> SNASFRVVLDPGHGGIDGGARGVTGILEKDVTLAFARALRDELQKGSHTIVALTRDSDIFLRLSERVKKAQEFDADLFISIHADTIDVHSLRGATVYTISDEASDAIAKSLAESENKVDLLDGLPKEESLELTDILLDLTRRETHAFSINFANNVVSNLSKSHINLINNPHRYADFQVLKAPDVPSVLIEIGYLSNKEDEKLLNNPQWRKQMAASIAYS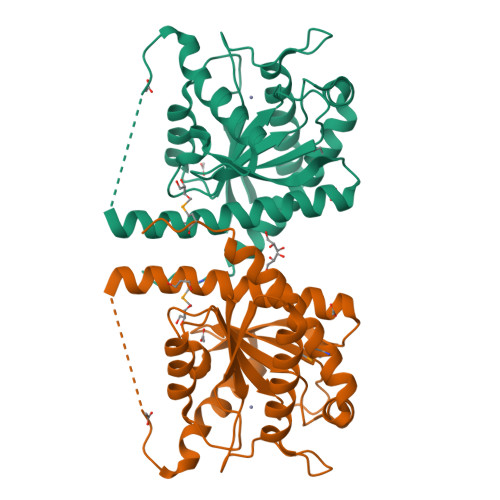IRQFAEYRQKIMQPL> MQDADKLPHTKVTLVAPPQVHPHEQATKSGPKVVEFTMTIEEKKMVIDDKGTTLQAMTFNGSMPGPTLVVHEGDYVQLTLVNPATNAMPHNVDFHGATGALGGAKLTNVNPGEQATLRFKADRSGTFVYHCAPEGMVPWHVVSGMSGTLMVLPRDGLKDPQGKPLHYDRAYTIGEFDLYIPKGPDGKYKDYATLAESYGDTVQVMRTLTPSHIVFNGKVGALTGANALTAKVGETVL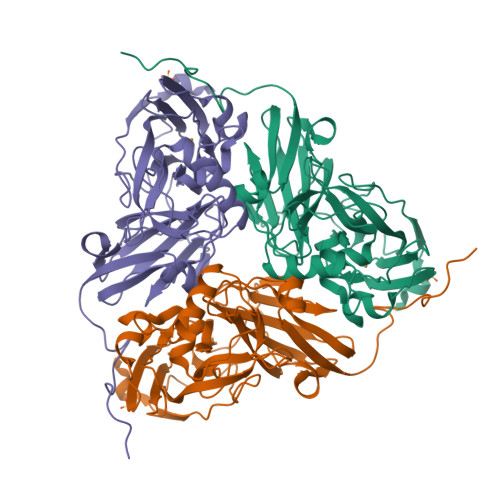LIHSQANRDTRPHLIGGHGDWVWETGKFANPPQRDLETWFIRGGSAGAALYTFKQPGVYAYLNHNLIEAFELGAAGHIKVEGKWNDDLMKQIKAPAPIPR Methylation catalysed by catechol-O-methyltransferase (COMT) is the main pathway of catechol neurotransmitter deactivation in the prefrontal cortex. COMT is a single-domain Mg2+-dependent methyltransferase that catalyses the transfer of an activated methyl group from S-adenosylmethionine (SAM) to its catechol substrate. The crystal structure of COMT comprises a central β-sheet flanked by α-helices, constructing a bipartite active site that accommodates the methyl donor SAM (in the so-called adenine site) and that can also complex an Mg2+ ion to which the catechol substrates bind. Here, a set of apo, semi-holo, holo and Michaelis form crystal structures are described that define the conformational space available to COMT and that include likely intermediates along the catalytic pathway.

A potential problem for in vivo data gained from mouse models that are not transgenic for human COMT is differences in the structures or activities of the homologues. In order to assure that the binding mode of compounds to mouse COMT is the same as that for rat and human COMT, it was hoped to determine a number of mouse COMT crystal structures in complex with selected inhibitors. However, in our hands mouse COMT proved to be difficult to crystallize and only an apo structure was obtained. However, when comparing this apo form with a human COMT apo structure, three loop regions that adopt different conformations in human and mouse COMT are identified. In human COMT the α2/α3 loop is disordered, but it is well defined in mouse COMT. Loop regions β5/α9 and β6/β7 are well defined but differ by distances of up to 8 Å at their tips. Importantly, in the mouse COMT structure these three loop regions adopt the same conformations as in the rat COMT structures and (see below). While it is possible that the apo state of COMT can adopt several conformations owing to an absence of conformational restrictions on the active-site loops, the recurrence of the same state in rat and mouse COMT points to a stable state of this apo form that is independent of crystal form and organism and that therefore may be adopted by COMT during catalysis after the reaction products have dissociated.

> MGGTKEQRILRHVQQHAKPGDPQSVLEAIDTYCSEKEWAMNVGDAKGQIMDAVIREYRPSLVLELGAYCGYSAVRMARLLPPGARLLTMEINPDYAAITQQMLDFAGLQDKVSILIGAPQDLIPQLKKKYDVDTLDMVFLDHWKDRYLPDTLLLEECGLLRKGTVLLADNVIVPGTPDFLAYVRGSSSFECTHYSSYLEYMKVVDGLEKAVYQGPGSSPVKS Here, we present a novel polymer-based support and an associated deposition method, with the aim of providing ultralow-background conditions for serial data collection. The supports themselves consist of a thin 2–3 µm thick cyclic olefin co­polymer (COC) membrane perforated with a dense array of 2–3 µm sized holes and suspended on a rigid frame. To assess the quality of structures that can be obtained from chip-mounted crystals, diffraction data were collected from a range of proteins. These proteins included the insulin, thaumatin and HEWL that were used in initial tests, and also TD1, a tubulin–DARPin D1 complex, EcR2a, a class Ia ribo­nucleotide reductase radical-generating subunit, rhodopsin–miniGo and PepTst, a bacterial peptide transporter.

TD1 and EcR2a are both soluble proteins with crystals grown using vapor diffusion, rhodopsin–miniGo is a membrane protein with crystals grown in vapor-diffusion plates and PepTst is a membrane protein where crystals are obtained using LCP methods. The deposition method was carefully studied using a variety of cases, including the lipid sponge phase, which is notoriously difficult to extract crystals from. However, successful blotting of sponge phase was demonstrated, offering new possibilities for handling and background reduction for sponge-phase samples. Blotting of the sponge phase was successful on the silanized chips; as shown by investigation of the background signal. This allowed a membrane-protein data set to be collected from the visible crystals. However, the procedure for sponge-phase blotting still requires substantial improvements and is not yet suitable for crystals that exist in both the cubic and sponge phase, which is a common occurrence in LCP crystallization trials. When a surfactant is present, i.e. for lipid- or detergent-containing crystallization buffers, the wetting on the polymer film is usually sufficient. In this respect, the chips presented here represent an attractive alternative delivery method for sponge-phase-grown crystals.

> MEDKGKTFFGQPLGLSTLFMTEMWERFSYYGMRAILLYYMWFLISTGDLHITRATAASIMAIYASMVYLSGTIGGFVADRIIGARPAVFWGGVLIMLGHIVLALPFGASALFGSIILIIIGTGFLKPNVSTLVGTLYDEHDRRRDAGFSIFVFGINLGAFIAPLIVGAAQEAAGYHVAFSLAAIGMFIGLLVYYFGGKKTLDPHYLRPTDPLAPEEVKPLLVKVSLAVAGFIAIIVVMNLVGWNSLPAYINLLTIVAIAIPVFYFAWMISSVKVTSTEHLRVVSYIPLFIAAVLFWAIEEQGSVVLATFAAERVDSSWFPVSWFQSLNPLFIMLYTPFFAWLWTAWKKNQPSSPTKFAVGLMFAGLSFLLMAIPGALYGTSGKVSPLWLVGSWALVILGEMLISPVGLSVTTKLAPKAFNSQMMSMWFLSSSVGSALNAQLVTLYNAKSEVAYFSYFGLGSVVLGIVLVFLSKRIQGL;> AF>GDLVFRQLAPNVWQHTSYLDMPGFGAVASNGLIVRDGGRVLVVDTAWTDDQTAQILNWIKQEINLPVALAVVTHAHQDK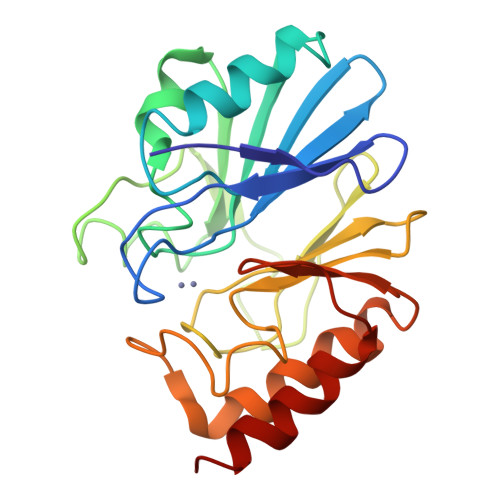MGGMDALHAAGIATYANALSNQLAPQEGMVAAQHSLTFAANGWVEPATAPNFGPLKVFYPGPGHTSDNITVGIDGTDIAFGGCLIKDSKAKSLGNLGDADTEHYAASARAFGAAFPKASMIVMSHSAPDSRAAITHTARMADKLR[2x]> MVQVEKGHVAVVFLNDPERRNPLSPEMALSLLQALDDLEADPGVRAVVLTGRGKAFSAGADLAFLERVTELGAEENYRHSLSLMRLFHRVYTYPKP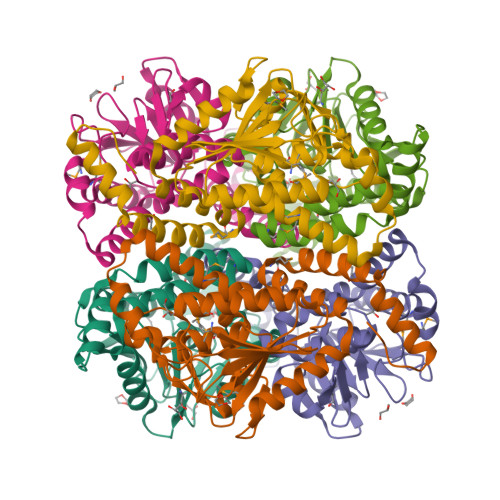TVAAVNGPAVAGGAGLALACDLVVMDEEARLGYTEVKIGFVAALVSVILVRAVGEKAAKDLLLTGRLVEAREAKALGLVNRIAPPGKALEEAKALAEEVAKNAPTSLRLTKELLLALPGMGLEDGFRLAALANAWVRETGDLAEGIRAFFEKRPPRF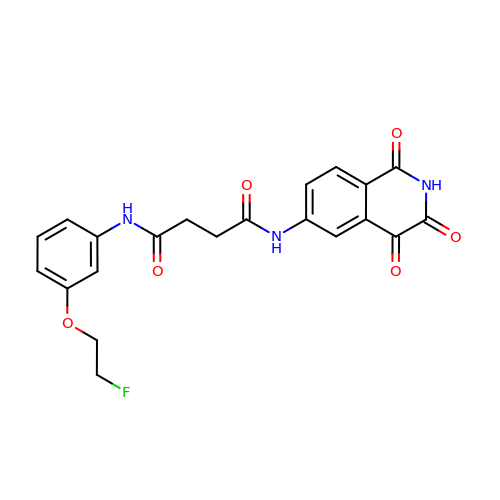N-[3-(2-fluoroethoxy)phenyl]-N'-(1,3,4-trioxo-1,2,3,4-tetrahydroisoquinolin-6-yl)butanediamide | C21 H18 F N3 O6 | DQXBKUVWJSZHSI-UHFFFAOYSA-N>MAGAAAAVTVEEVRKAQRASGPATVLAIGTATPANCVHQADYPDYYFRVTKSDHLTDLKEKFKRMCDKSMIRKRYMHLTEEFLAENPNMCAYMAPSLDARQDIVVVEVPKLGKAAAQKALKEWGQPRSRITHLVFCTTSGVDMPGADYQLTKLLGLRPSVNRLMMYQQGSFAGGTVLRVAKDLAENNRGARVLVVCSEITAVTFRGPSESHLDSLVGQALFGDGAAAVIVGADPDERAERPLFQLVSAAQTLLPDSEGAIDGHLREVGLTFHLLKDVPGLISKNIERALEAAFAPLGISDWNSIFWVAHPGGPAILDQVEAKVSLDKARMRATRHVLAEYGNMSSACVLFILDEMRKRSAEDGCATTGEGLDWGVLFGFGPGLTVETVVLHSVPITAGAAAA[2x]

Chalcone synthase (CHS) and chalcone isomerase (CHI) catalyze the first two committed steps of the flavonoid pathway that plays a pivotal role in the growth and reproduction of land plants, including UV protection, pigmentation, symbiotic nitrogen fixation, and pathogen resistance. Based on the obtained X-ray crystal structures of CHS, CHI, and chalcone isomerase-like protein (CHIL) from the same monocotyledon, Panicum virgatum, along with the results of the steady-state kinetics, spectroscopic/thermodynamic analyses, intermolecular interactions, and their effect on each catalytic step are proposed. The production of these value-added products also offers the prospect of increasing the value of the crop, especially because many of these compounds are soluble and readily extracted. This study characterized the enzymes involved in the first two committed steps of the flavonoid pathway, CHS and CHI, and the non-catalytic protein CHIL. Through crystal structure, molecular docking, mutagenesis, kinetic analyses, ITC, and FRET analysis, our study provides evidence supporting a revised catalytic reaction mechanism for monocot CHS and CHI and identified an intermolecular interaction of CHS with both CHI and CHIL in a non-competitive manner.

The C170S mutant PvCHS was generated to investigate its potential impact on the local conformation and confirm the catalytic role. The asymmetric unit contained two mutant PvCHS molecules, as observed in the wild-type PvCHS. The overall RMSD between the mutant C170S and the WT PvCHS was small, with 0.26 Å. Importantly, the catalytic triad remained stable with a distance of 4.49 Å (3.2 Å in wild type) between the Ser-170 hydroxyl group and Asn-342 carboxamide and 5.57 Å (vs. 3.2 Å) between the serine hydroxyl and the Asn-342 carboxamide. Nε2 of His-309 was 3.84 Å (vs. 3.2 Å). The noticeable changes in distances are associated with the shorter sidechain group of serine than the oxidized cysteine.> GAGHMASPSENLSRKAKKKAIQQSPEALLKQKLDMCSKKGDVLEALRLYDEARRNGVQLSQYHYNVLLYVCSLAEAATESSPNPGLSRGFDIFKQMIVDKVVPNEATFTNGARLAVAKDDPEMAFDMVKQMKAFGIQPRLRSYGPALFGFCRKGDADKAYEVDAHMVESEVVPEEPELAALLKVSMDTKNADKVYKTLQRLRDLVRQVSKSTFDMIEEWFKSEVATKTGVKKWDVKKIRDAVVSGGGGWHGQGWLGTGKWNVKRTEMDENGVCKCCKEKLVCIDINPVETETFAASLTRLACEREVKANFNQFQEWLERHGPFDAVIDGANMGLVNQRSFSFFQLNNTVQRCQQISPSKRLPLVILHKSRVNGGPATYPKNRALLEKWKNAGALYATPPGSNDDWYWLYAAVSCKCLLVTNDEMRDHLFQLLGNSFFPRWKEKHQVRISVTREDGLKLNMPPPYSIVIQESEDGTWHVPM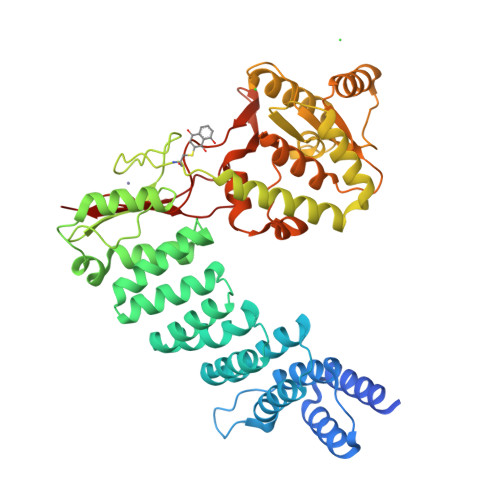SVEDDLQTSRQWLCAKRSKTP> APLATRQGKRPSKNLKARCSRKALHVNFKDMGWDDWIIAPLEYEAFHCEGLCEFPLRSHLEPTNHAVIQTLMNSMDPESTPPT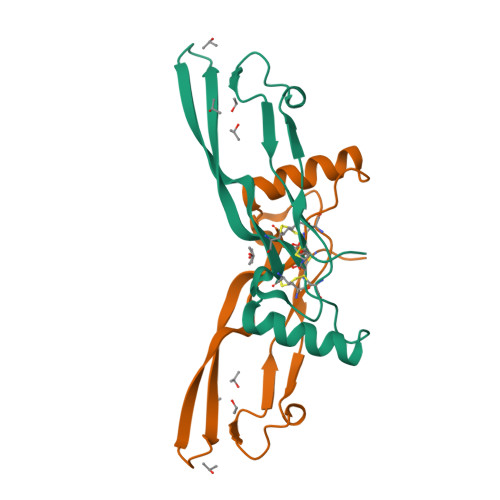CCVPTRLSPISILFIDSANNVVYKQYEDMVVESCGCR Here, we report the three-dimensional structure of a ‘Termamyl’-like α-amylase, the AliC α-amylase from Alicyclobacillus sp. 18711. One particularly important subset of GH13 enzymes are the ‘Termamyl’-like α-amylases, historically named after an enzyme from Bacillus licheniformis. These enzymes typically feature a three-domain ‘A, B, C’ arrangement with a C-terminal β-sheet domain and with domain B being a protrusion from the (β/α)8 fold of domain A. The catalytic centre is placed in domain A, whilst the A–B interface forms the substrate-binding cleft. The fold, as expected, is a canonical three-domain arrangement with the A, B and C domains defined approximately as A, residues 4–104 and 210–397; B, residues 105–209; and C, residues 398–484. A classical Ca2+–Na+–Ca2+ triad is found at the A/B-domain interface.

In order to try and access a branched complex with a branch in the +1 subsite (the position of which is harder to model from the 6-deoxy sugars present in acarbose alone) we sought to obtain a complex by co-crystallizing AliC with 63-α-d-glucosyl maltotriose (Megazyme, Wicklow, Ireland) and observing what was obtained with this active enzyme. A ‘branched-ligand’ AliC complex was obtained through co-crystallization, with crystals forming in a new space group. This form diffracted poorly and data could only be obtained to 2.95 Å resolution. A subsequent lower resolution (approximately 3 Å) analysis revealed the binding of a branched ligand in the +1/+2 subsites with an α-1,6-linked glucose branch bound to the +1 subsite sugar. Weak density in the −1 subsite, largely diffuse but greater than would be expected for discrete solvent, remained unmodelled. Notably, this +1′ sugar overlaps in position with the very recently reported SusG amylase branched-ligand complex. The accommodation of branch points was therefore investigated by an analysis of limit digestion products (the characteristic oligosaccharides remaining after enzymatic digestion) on both pullulan (a regular linear polysaccharide of α-1,4, α-1,4, α-1,6 repeating trisaccharides) and amylopectin, an α-1,6-branched starch structure. The action of AliC on pullulan results in the production of the trisaccharide panose, glucose α-1,6-glucose α-1,4-glucose, demonstrating that the enzyme must be able to accommodate α-1,6 linkages to glucose moieties in both the +1 and −2 subsites.

>TFAGDNGTMMQYFEWYLPNDGTLWTKMGSDASHLKSIGITGVWFPPAYKGQSQSDVGYGVYDMYDLGEFNQKGTVRTKYGTKAQLQSAITSLHNNGIQAYGDVVLNHRMGADATETISAVEVNPSNRNQVTSGAYNISAWTDFEFPGRGNTYSSFKWHSYYFDGVDWDQSRQLSGKIYQIQGKAWDWEVDSENGNYDYLMGADIDYDHPDVQTEVKNWGKWFVNTLNLDGVRLDAVKHIKFDYMSSWLSSVKSTTGKSNLFAVGEYWNTSLGALENYENKTNWSMSLFDVPLHMNFQAAANGGGYYDMRNLLNNTMMKNHPIQAVTFVDNHDTEPGQALQSWVSDWFKPLAYATILTRQEGYPCVFYGDYYGIPSQSVSAKSTWLDKQLSARKSYAYGTQHDYLDNQDVIGWTREGDSAHAGSGLATVMSDGPGGSKTMYVGTAHAGQVFKDITGNRTDTVTINSAGNGTFPCNGGSVSIWVKQ[4x]>ASCLELALEGERLCKSGDCRAGVSFFEAAVQVGTEDLKTLSAIYSQLGNAYFYLHDYAKALEYHHHDLTLARTIGDQLGEAKASGNLGNTLKVLGNFDEAIVCCQRHLDISRELNDKVGEARALYNLGNVYHAKGKSFGCPGPQDVGEFPEEVRDALQAAVDFYEENLSLVTALGDRAAQGRAFGNLGNTHYLLGNFRDAVIAHEQRLLIAKEFGDKAAERRAYSNLGNAYIFLG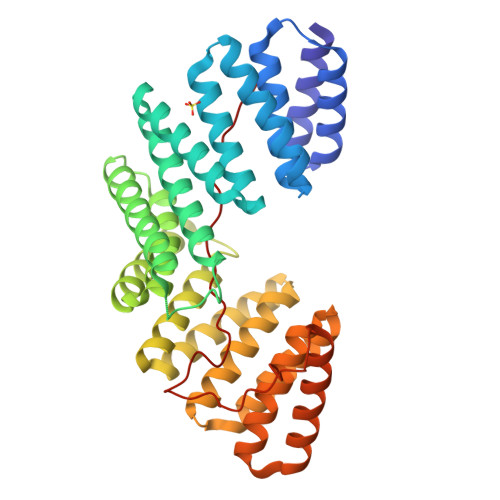EFETASEYYKKTLLLARQLKDRAVEAQSCYSLGNTYTLLQDYEKAIDYHLKHLAIAQELNDRIGEGRACWSLGNAYTALGNHDQAMHFAEKHLEISREVGDQRNASYLKTQVLSPDSLFTAKFVAYNEEEEEEDCSLAG[2x]> APAVPDKPVEVKGSQKTVMFPHAPHEKVECVTCHHLVDGKESYAKCGSSGCHDDLTAKKGE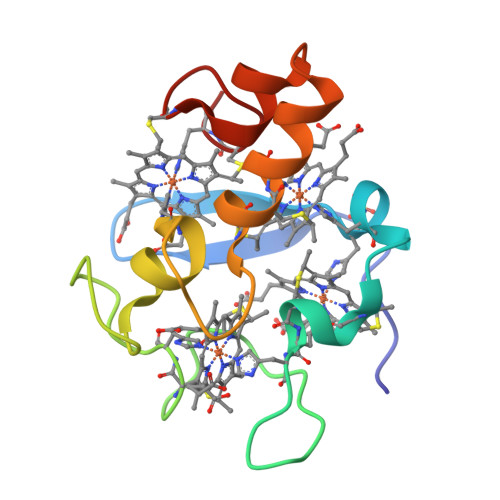KSLYYVVHARGELKHTSCLACHSKVVAEKPELKKDLTGCAKSKCHP> 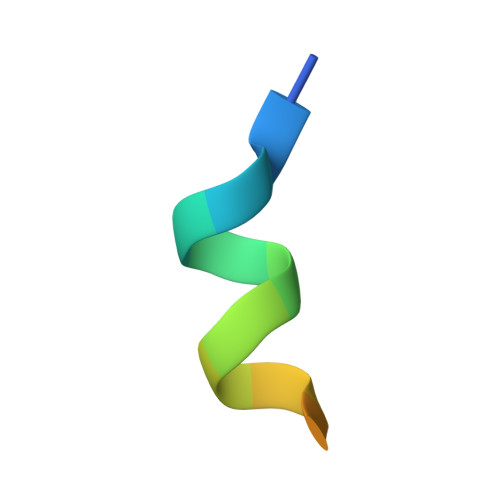EFPYLLSLLGEVSPQ Prenyltransferases, also known as isoprenyl diphosphate synthases, catalyze the sequential condensation of a basic five-carbon building block (C5), the isopentenyl diphosphate (IPP), to synthesize prenyl precursors of isoprenoid metabolites and isoprene polymers, collectively called polyisoprene. Ultrahigh molecular weight cis-1,4-polyisoprene and trans-1,4-polyisoprene (TPI), which are the principal components of natural rubber and gutta-percha, respectively, are also isoprenoid metabolites that are assumed to be synthesized by specialized prenyltransferases. These prenyltransferases are divided into two major groups, the cis-1,4-prenyltransferases (CPTs) and trans-1,4-prenyltransferases (TPTs), based on the stereochemistry of the double bond formed during IPP condensation. To investigate the molecular properties of the EuTPT proteins, we determined the three-dimensional structures of EuTPT3 and EuFPS1 using X-ray crystallography. Similar to EuFPS1 and other prenyltransferases, the EuTPT3 subunits were composed of 10 core helices (α1-α10) with a deep pocket that included two DDxxD motifs responsible for substrates binding.

It should be noted that we previously characterized EuTPT2 and EuTPT4 as E. ulmoides FPS proteins, referred to as EuFPS1 and EuFPS2, respectively. In the tetrad analysis, ScFPS, EuTPT2, and EuTPT4 rescued Δfps lethality. The superimposition parameters suggested that the dimeric architecture of EuTPS3 was highly conserved and unlikely to be caused by crystal packing. Interestingly, the dimeric architecture of EuTPT3 substantially differed from that of EuFPS1, which formed a conventional TPT dimer. In EuTPT3, α6 of one subunit interacted with α5 and α6 of the neighboring subunit to form a four-helix bundle, whereas, in EuFPS1, α4 of one subunit was inserted between α5 and α6 of the neighboring subunit to form a six-helix bundle of α4–α6 at the dimer interface. As a result, the neighboring subunit of EuFPS1 was tilted at an angle of ~45° compared with that of EuTPT3. The structural difference is related to the chain length determination residues, which are conserved as bulky amino acids among FPSs, including EuFPS1 and 2. Specifically, the equivalent positions of residues Cys94 and Ala95 on α4 in EuTPT3 are occupied by Tyr88 and Phe89 in EuFPS1. The side chains of those residues protrude between α5 and α6, resulting in a marked bending of α5. The residues equivalent to Tyr88 and Phe89 in EuFPS1 are highly conserved among all FPSs. The TPT-type dimer formed a larger hollow at the dimer interface and supported a hydrophobic tunnel reaching through the bottom region, whereas the bulky side chains of Tyr88 and Phe89 appeared to prevent the formation of a tunnel in EuFPS1.

>[2x]MNHKVHHHHHHIEGRHMSDLKSKFLEVYSVLKSELLNDPAFDFTDDSRLWVERMLDYNVPGGKLNRGLSVIDSFKLLKEGKEPTDEEIFLACVLGWCIEWLQAYFLVLDDIMDSSHTRRGQPCWFRLPKVGMIAVNDGLILRNHIPRILKKHFKGKPYYVDLLDLFNEVEFQTASGQMIDLITTLVGEKDLSKYSLPLHHRIVQYKTAYYSFYLPVACALVMSGENLDNHVDVKNILVEMGTYFQVQDDYLDCFGDPKFIGKIGTDIEDFKCSWLVVKALELANDEQKKLLHENYGKEDPECVAKVKKLYETLNLQDVFGEYERQSHGKLIKAIEGHSNKAVQFVLKSSLEKIYQRQK> SSYAGPATWYEGNVAGGTCSFSGYTLAPGIFGTALTDSSWSDAAHCGACISVKGPSGNSIKVMIVDECPGCGTNHLDLFEDAFAQLAATSVGVINVDWSFVPCGIDTPITLKNKDGTSAYWFSMQVV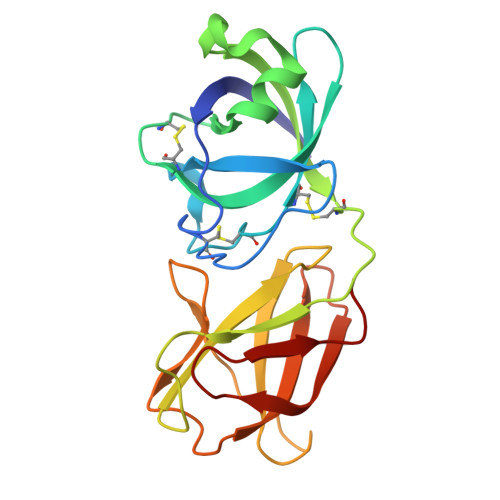NANEPVASLEVSTDGGSTWQSTTRTYYNYFEKQSGFGTDTVDVRITSTSGATITVKNVSCQSESTTTASSNF(1S)-5-deoxy-1-O-methyl-1-C-[(2R,3S)-3,5,7,10-tetrahydroxy-6-methyl-4-oxo-1,2,3,4-tetrahydroanthracen-2-yl]-D-xylulose | C21 H24 O9 | 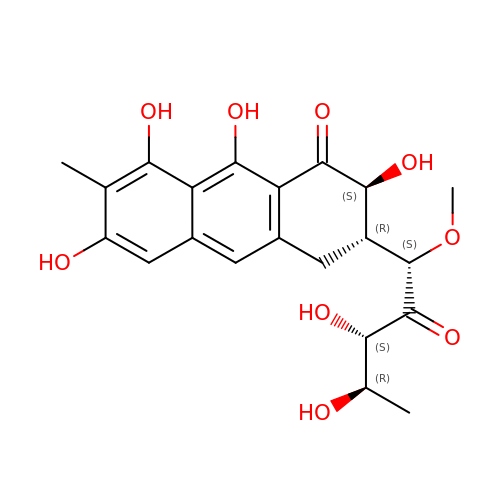AOCJXLJIUYHXRS-PKRZCTMMSA-N> MGVYDYKNFGTADSKALFSDAMAITLYSYHNLDNGFAAGYQHNGFGLGLPATLVT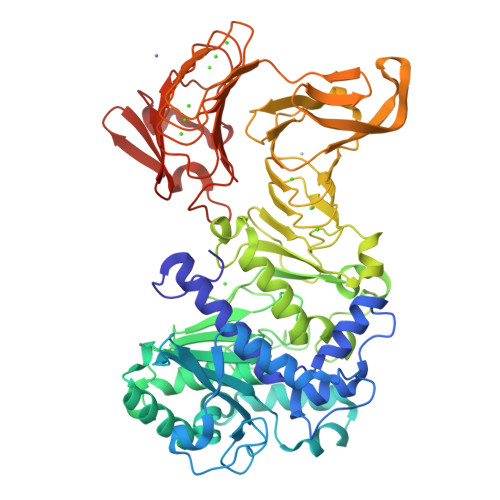ALLGGTDSQGVIPGIPWNPDSEKLALDAVKKAGWTPITASQLGYDGKTDARGTFFGEKAGYTTAQVEILGKYDAQGHLTEIGIAFRGTSGPRENLILDSIGDVINDLLAAFGPKDYAKNYVGEAFGNLLNDVVAFAKANGLSGKDVLVSGHSLGGLAVNSMADLSGGKWGGFFADSNYIAYASPTQSSTDKVLNVGYENDPVFRALDGSTFTGASVGVHDAPKESATDNIVSFNDHYASTAWNLLPFSILNIPTWISHLPTAYGDGMNRIIESKFYDLTSKDSTIIVANLSDPARANTWVQDLNRNAETHKGSTFIIGSDSNDLIQGGSGNDYLEGRAGNDTFRDGGGYNVILGGAGNNTLDLQKSVNTFDFANDGAGNLYVRDANGGICITRDIGSIVTKEPGFLWGLFKDDVTHSVTASGLKVGSNVTQYDASVKGTNGADTLKAHAGGDWLFGLDGNDHLIGGVGNDVFVGGAGNDLMESGGGADTFLFNGAFGQDRVVGFTSNDKLVFLGVQGVLPNDDFRAHASMVGQDTVLKFGGDSVTLVGVALNSLSADGIVIA> MQNEYLDAKKHGIDLSRERAPNFVDHPGIPPSDCFWFLYKNYVRQDAG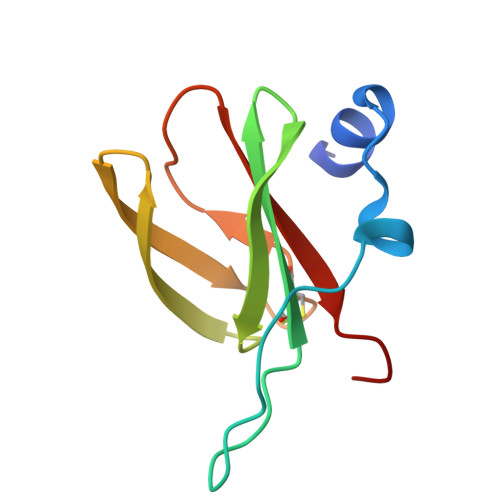VCQSDWSFDMKIGQYWVTIHTDEGCRLSGIIPAGWLILGIKRLGF> MSSAVEKKDLPADYGKMPAGYNFLTRGKDWREYDKDFILRTDAVWEKFQLEHFFRNYMKCFFFDHGLKKYQMFEPEDMYTVVFEGWALDDLITFPGFTPTGRTNSYQIGLSPRQRTVVPTQTFYQMQDYYMLCGLRFERWFRCDLVYHDQRHTKFDQVKNQKNYKTYPCYREYYEAQYACQDDMFDFLMELAYARRAADNFESDFASHELTTLPTF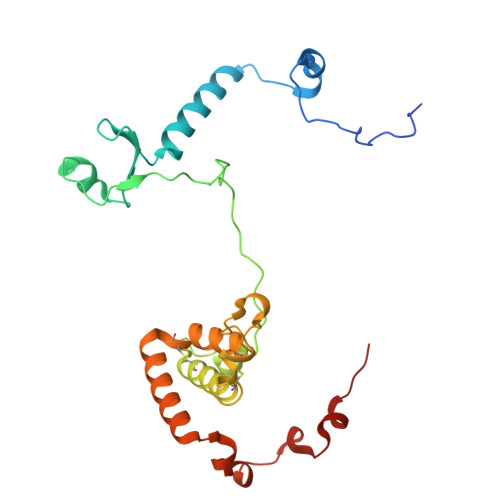YDTPKAAERKTYTY>[10x]MACLTDLVNLNLSDTTEKIIAEYIWIGGSGMDLRSKARTLPGPVTDPSKLPKWNYDGSSTGQAPGEDSEVILYPQAIFKDPFRRGNNILVMCDCYTPAGEPIPTNKRYSAAKIFSSPEVAAEEPWYGIEQEYTLLQKDTNWPLGWPIGGFPGPQGPYYCGIGAEKSFGRDIVDAHYKACLYAGINISGINGEVMPGQWEFQVGPSVGISSGDQVWVA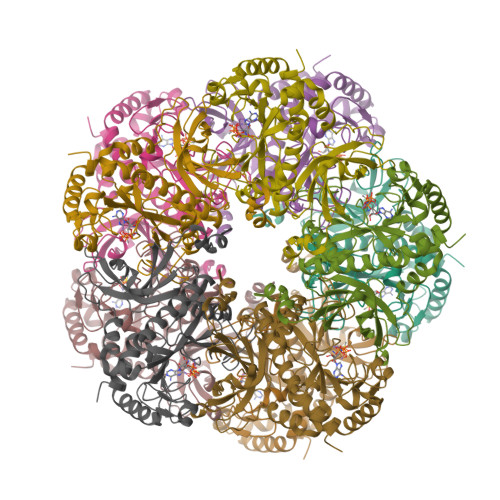RYILERITEIAGVVVTFDPKPIPGDWNGAGAHTNYSTESMRKEGGYEVIKAAIEKLKLRHKEHIAAYGEGNERRLTGRHETADINTFSWGVANRGASVRVGRETEQNGKGYFEDRRPASNMDPYVVTSMIAETTIVWKP>[4x]MVGLADVAVL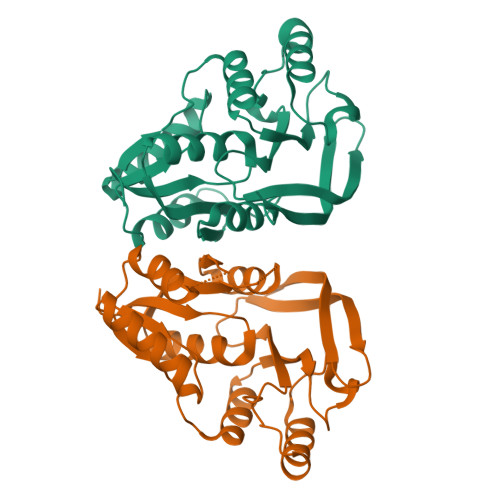YSGGKDSNYALYWALKSGLRVRYLVSMVSENEESYMYHTPNVELTSLQARALGIPIIKGFTKGEKEKEVEDLKNVLEGLKVDGIVAGALASRYQKERIENVARELGLKVYTPAWEKDPYQYMLEIIKLGFKVVFVAVSAYGLNESWLGRELNYKNLEELKKLSEKYGIHIAGEGGEFETFVLDMPFFKAKIVIDDAEKFWDGLSGKFIIKRAHLEWK> HHHHHHGSDPIHYDKITEEINKAIDDAIAAIEQSETIDPMKVPDHADKFERHVGILDFKGELAMRNIEARGLKQMKRQGDANVKGEEGIVKAHLLIGVHDDIVSMEYDLAYKLGDLHPTTHVISDIQDFVVALSLEIPDEGNITMTSFEVRQFANVVNHIGGLSILDPIFGVLSDVLTAIFQDTVRKEMTKVLAPAFKRE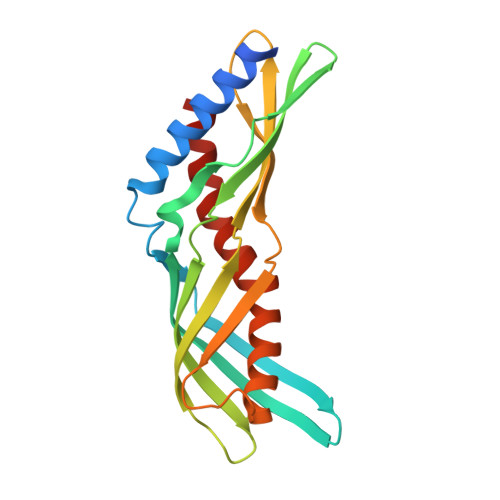LEKN>AMKNRALLLIDFQKGIESPTQQLYRLPAVLDKVNQRIAVYRQHHAPIIFVQHEETELPFGSDSWQLFEKLDTQPTDFFIRKTHANAFYQTNLNDLLTEQAVQTLEIAGVQTEFCVDTTIRMAHGLGYTCLMTPK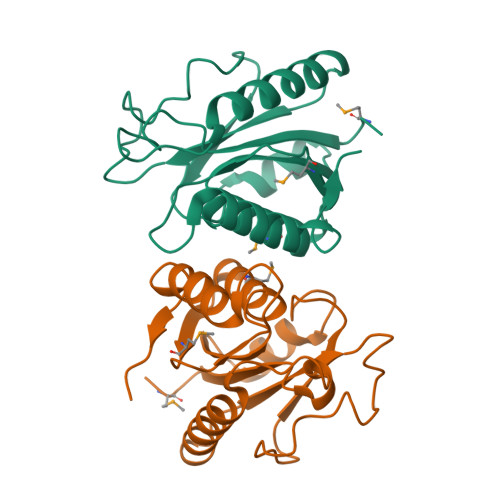TTSTLDNGHLTAAQIIQHHEAIWAGRFLTFLSL[4x]>[2x]MASHHHHHHGSMAEGEEYDKILVLNFGSQYFHLIVKRLNNIKIFS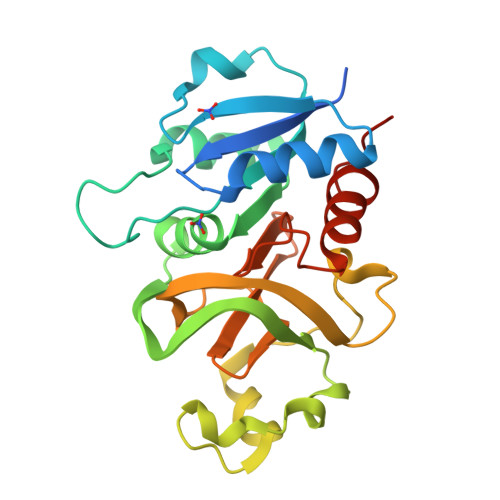ETKDYGVELKDIKDMNIKGVILSGGPYSVTEAGSPHLKKEVFEYFLEKKIPIFGICYGMQEIAVQMNGEVKKSKTSEYGCTDVNILRNDNINNITYCRNFGDSSSAMDLYSNYKLMNETCCLFENIKSDITTVWMNHNDEVTKIPENFYLVSSSENCLICSIYNKEYNIYGVQYHPEVYESLDGELMFYNFAYNICKCKKQFDP> LNEHTAGDTTKSPYTIYAGLGFAVQESCYYCHGNGGKGTTEGLIFGVPDFTSTEFQSSMTDKQIID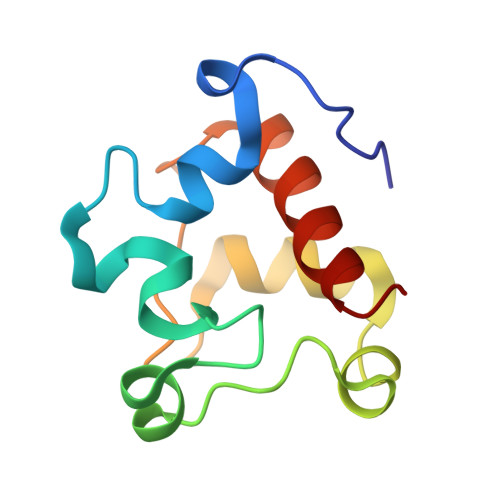HINKGKGKMPSYQGKMSPEMIEKMAGVVRNFAVK>[6x]AASAAPARPAHPLDPLSTAEIKAATNTVKSYFAGKKISFNTVTLREPARKAYIQWKEQGGPLPPRLAYYVILEAGKPGVKEGLVDLASLSVIETRALETVQPILTVEDLCSTEEVIRNDPAVIEQCVLSGIPANEMHKVYCDPWTIGYDERWGTGKRLQQALVYYRSDEDDSQYSHPLDFCPIVDTEEKKVIFIDIPNRRRKVSKHKHANFYPKHMIEKVGAMRPEAPPINVTQPEGVSFKMTGNVMEWSNFKFHIGFNYREGIVLSDVSYNDHGNVRPIFHRISLSEMIVPYGSPEFPHQRKHALDIGEYGAGYMTNPLSLGCDCKGVIHYLDAHFSDRAGDPIT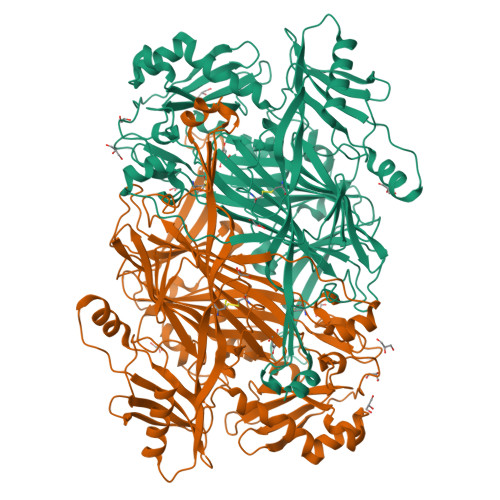VKNAVCIHEEDDGLLFKHSDFRDNFATSLVTRATKLVVSQIFTAANYEYCLYWVFMQDGAIRLDIRLTGILNTYILGDDEEAGPWGTRVYPNVNAHNHQHLFSLRIDPRIDGDGNSAAACDAKSSPYPLGSPENMYGNAFYSEKTTFKTVKDSLTNYESATGRSWDIFNPNKVNPYSGKPPSYKLVSTQCPPLLAKEGSLVAKRAPWASHSVNVVPYKDNRLYPSGDHVPQWSGDGVRGMREWIGDGSENIDNTDILFFHTFGITHFPAPEDFPLMPAEPITLMLRPRHFFTENPGLDIQPSYAMTTSEAKRAV> GSMAQEQTKRGGG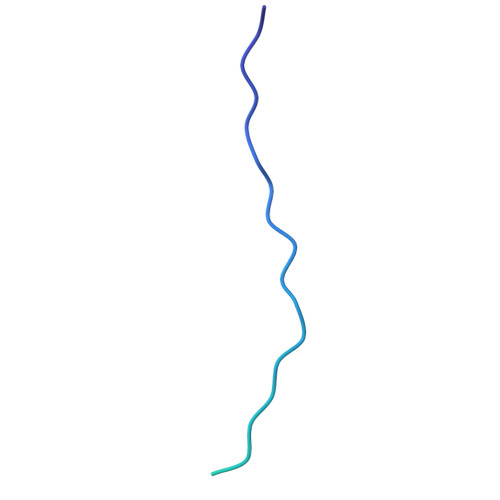GGDDDDIAGSTAAGQERREKLTEETDDLLDEIDDVLEENAEDFVRAYVQKGGQ>RTRQLQQLQDAVIEALATLGDLRDNPRSRHLPRIERYVRLLAEHLAAQRAFADELTPEAVDLLSKSALLHDIGKVAVPDRVLLNPGQLDAADTALLQGHTRAGRDALASAERRLGQPSGFLRFARQIAYSHHERWDGRGFPEGLAGERIPLAARIVAL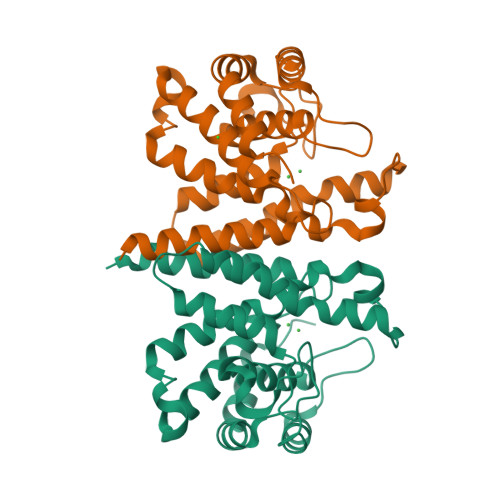ADRYDELTSRHAYRPPLAHAEAVLLIQAGAGSEFDPRLVEAFVAVADAFAEVARRYADSA[2x]> MLRRFPTRTTAPGQGGARRSRVRALAWLLASGAMTHLSPALADVPYVLVKTNMVVTSVAMKPYEVT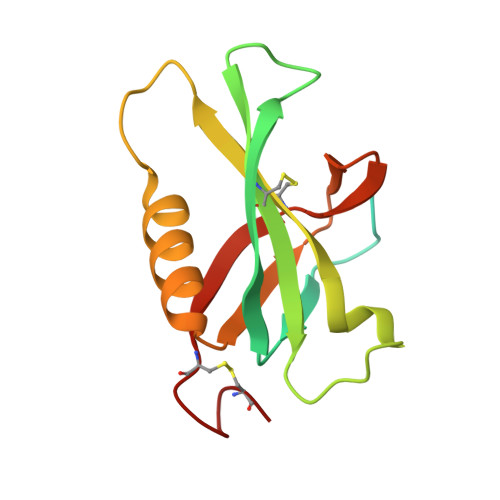PTRMLVCGIAAKLGAAASSPDAHVPFCFGKDLKRPGSSPMEVMLRAVFMQQRPLRMFLGPKQLTFEGKPALELIRMVECSGKQDCP> ISFRQQPEENACQFQRLNAQRP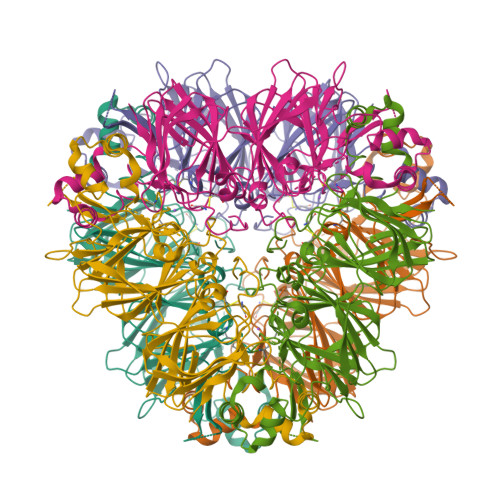DNRIESEGGYIETWNPNNQEFECAGVALSRLVLRRNALRRPFYSNAPQEIFIQQGRGYFGLIFPGCPSTYEEPAQQGRRYQSQRPPRRLQEEDQSQQQQDSHQKVHRFNEGDLIAVPTGVAFWLYNDHDTDVVAVSLTDTNNNDNQLDQFPRRFNLAGNHEQEFLRYQQQSRQSRRRSLPYSPYSPQSQPRQEEREFSPRGQHSRRERAGQEEEHEGGNIFSGFTPEFLAQAFQVDDRQIVQNLRGENESEEQGAIVTVRGGLRILSPDRKRGADEEEEYDEDEYEYDEEDRRRGRGSRGSGNGIEETICTATVKKNIGRNRSPDIYNPQAGSLKTANELNLLILRWLGLSAEYGNLYRNALFVPHYNTNAHSIIYALRGRAHVQVVDSNGNRVYDEELQEGHVLVVPQNFAVAGKSQSDNFEYVAFKTDSRPSIANLAGENSVIDNLPEEVVANSYGLPREQARQLKNNNPFKFFVPPSQQSPRAVA>[2x]SLELLEPPTQMRDLTASQLLDEITIGWNLGNTLDATTTSWLPNPTPAQSETAWGCPMTTKAMIDKVKEGGFNTVRVPVSWIDHTGSAPEYQIDEAWMNRVQEVVNYVIDNDMYCILNIHHENDWLIPTNAQK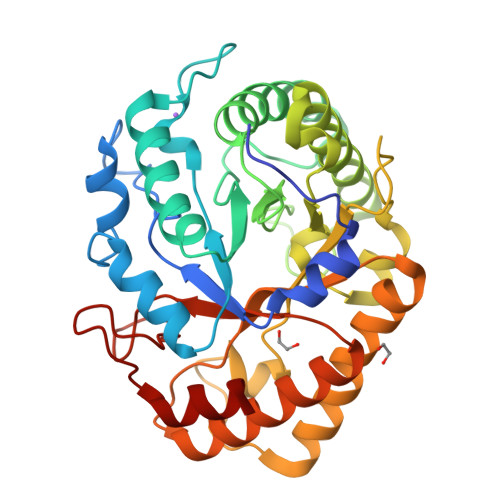DSVNARLDAIWTQIATRFGSYDEHLIFEGMNQPRLVGDPNEWNGGNQEARQVINSYNQTFVNTVRATGGNNAIRCLMVPTYAASCSSTTVNDFVLPTDTVANKLIVDIHSYSPYNFALNTSGTSSFTQSDISQLQWTLQEIYNSFGAKGIPVIIGQFGALNKNNINGRVLWGENYLRIAKSYNIRCIWWDNNAFDTSGENFGLLNRGTLTWQYPELLEAMMK> TEAAAQPHALPADAPDIAPERDLLSKFDGLIAERQKLLDSGVTDPFAIVMEQVKSPTEAVIRGKDTILLGTYNYMGMTFDPDVIAAGKE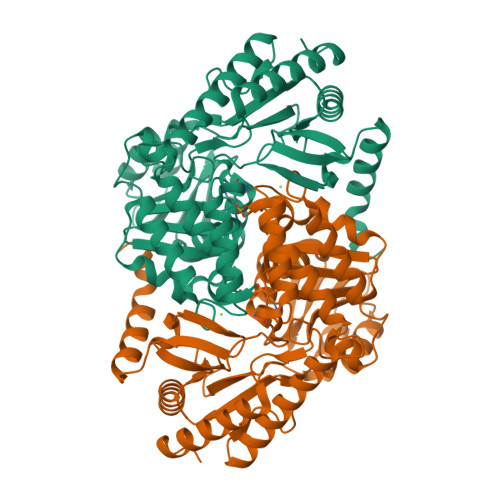ALEKFGSGTNGSRMLNGTFHDHMEVEQALRDFYGTTGAIVFSTGYMANLGIISTLAGKGEYVILDADSHASIYDGCQQGNAEIVRFRHNSVEDLDKRLGRLPKEPAKLVVLEGVYSMLGDIAPLKEMVAVAKKHGAMVLVDEAHSMGFFGPNGRGVYEAQGLEGQIDFVVGTFSKSVGTVGGFVVSNHPKFEAVRLACRPYIFTASLPPSVVATATTSIRKLMTAHEKRERLWSNARALHGGLKAMGFRLGTETCDSAIVAVMLEDQEQAAMMWQALLDGGLYVNMARPPATPAGTFLLRCSICAEHTPAQIQTVLGMFQAAGRAVGVIGLEHHHHHH>GSQQIKDPLNYEVEPFTFQNQDGKNVSLESLKGEVWLADFIFTNCETICPPMTAHMTDLQKKLKAENIDVRIISFSVDPENDKPKQLKKFAANYPLSFDNWDFLTGYSQSEIEEFALKSFKAIVKKPEGEDQVIHQSSFYL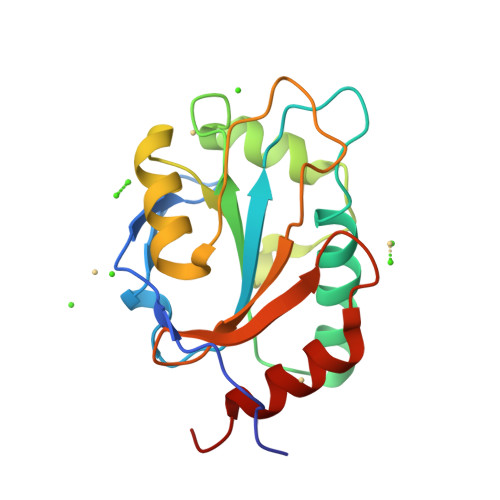VGPDGKVLKDYNGVENTPYDDIISDVKSASTLK[2x]(2R,6S)-2-amino-6-(carboxyamino)-7-{[(1R)-1-carboxyethyl]amino}-7-oxoheptanoic acid | C11 H19 N3 O7 | 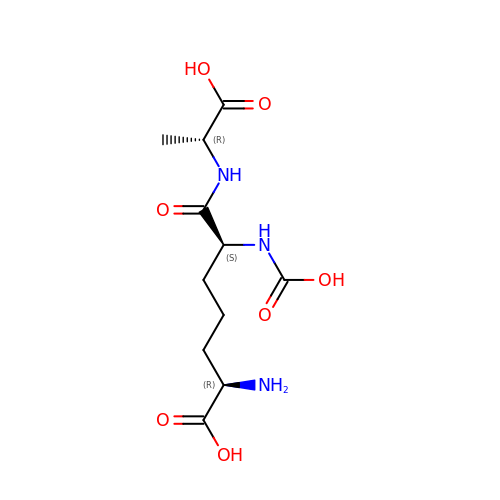HUCJTZSCCQLPOD-QYNIQEEDSA-N>[2x]MAIRLYKLAVALGVFIVSAPAFSHGHHSHGKPLTEVEQKAANGVFDDANVQNRTLSDWDGVWQSVYPLLQSGKLDP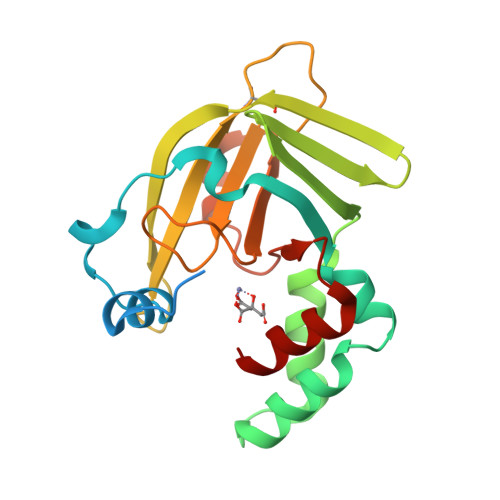VFQKKADADKTKTFAEIKDYYHKGYATDIEMIGIEDGIVEFHRNNETTSCKYDYDGYKILTYKSGKKGVRYLFECKDPESKAPKYIQFSDHIIAPRKSSHFHIFMGNDSQQSLLNEMENWPTYYPYQLSSEEVVEEMMSH> QIPLCANLVPVPITNATLDQITGKWFYIASAF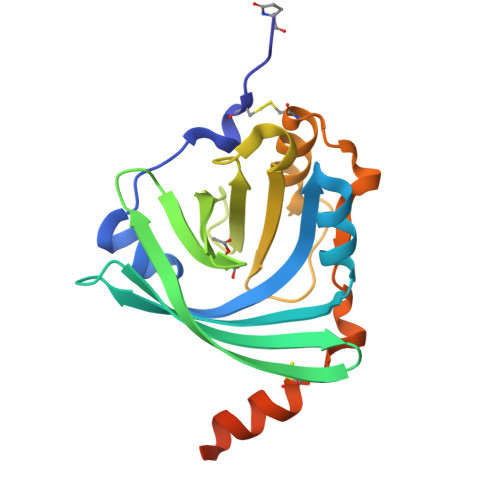RNEEYNKSVQEIQATFFYFTPNKTEDTIFLREYQTRQDQCIYNTTYLNVQRENGTISRYVGGQEHFAHLLILRDTKTYMLAFDVNDEKNWGLSVYADKPETTKEQLGEFYEALDCLRIPKSDVVYTDWKKDKCEPLEKQHEKERKQEEGESAWSHPQFEK>MNPVHILAKKGEVAERVLVVGDPGRARLLSTLLQNPKLTNENRGFLVYTGKYNGETVSIATHGIGGPSIAIVLEELAMLGANVFIRYGTTGALVPYINLGEYIIVTGASYNQGGLFYQYLRDNACVASTPDFELTNKLVTSFSKRNLKYYVGNVFSSDAFYAEDEEF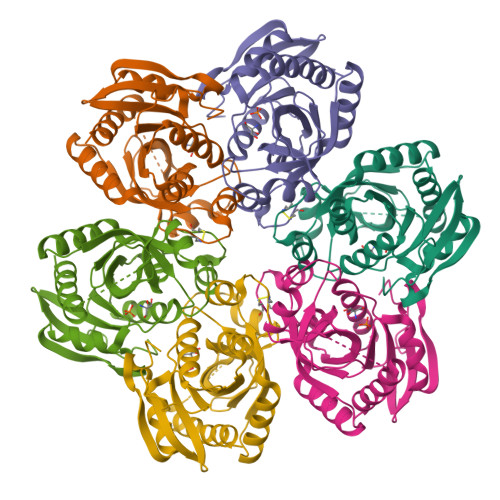VKKWSSRGNIAVEMECATLFTLSKVKGWKSATVLVVSDNLAKGGIWITKEELEKSVMDGAKAVLDTLTS[6x]>AMADITSLYKKAGSAAAPFAYNSAGEPPVSRRSFPKGFIFGTASSSYQYEGGAAEGGRGPSIWDTFTHQHPEKIADRSNGDVASDSYHLYKEDVRLMKDMGMDAYRFSISWTRILPNGSLRGGVNKEGIKYYNNLINELLSKGVQPFITLFHWDSPQALEDKYNGFLSPNIINDFKDYAEICFKEFGDRVKNWITFNEPWTFCSNGYATGLFAPGRCSPWEKGNCSVGDSGREPYTACHHQLLAHAETVRLYKAKYQA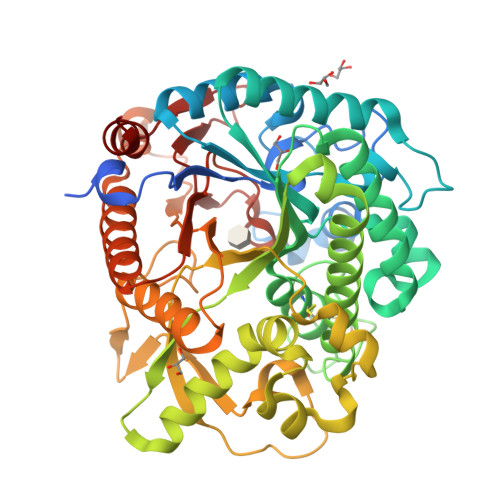LQKGKIGITLVSHWFVPFSRSKSNNDAAKRAIDFMFGWFMDPLIRGDYPLSMRGLVGNRLPQFTKEQSKLVKGAFDFIGLNYYTANYADNLPPSNGLNNSYTTDSRANLTGVRNGIPIGPQAASPWLYVYPQGFRDLLLYVKENYGNPTVYITENGVDEFNNKTLPLQEALKDDARIEYYHKHLLSLLSAIRDGANVKGYFAWSLLDNFEWSNGYTVRFGINFVDYNDGRKRYPKNSAHWFKKFLLK[2x]>[4x]MAIGYVWNTLYGWVDTGTGSLAAANLTARMQPISHHLAHPDTKRRFHELVCASGQIEHLTPIAAVAATDADILRAHSAAHLENMKRVSNLPTGGDTGDGITMMGNGGLEIA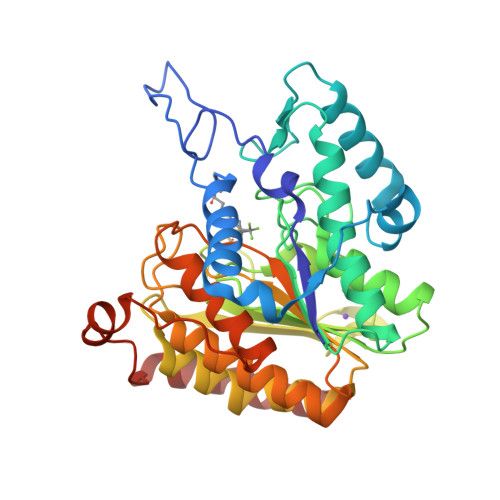RLSAGGAVELTRRVATGELSAGYALVNPPGHHAPHNAAMGFCIFNNTSVAAGYARAVLGMERVAILDWDVHHGNGTQDIWWNDPSVLTISLHQHLCFPPDSGYSTERGAGNGHGYNINVPLPPGSGNAAYLHAMDQVVLPALRAYRPQLIIVGSGFDASMLDPLARMMVTADGFRQMARRTIDCAADICDGRIVFVQEGGYSPHYLPFCGLAVIEELTGVRSLPDPYHEFLAGMGGNTLLDAERAAIEEIVPLLADIR> SLKPLTLLMTSSTSFSETINQWADILKTTDMEKFSFDSNPINLLELVKQFNLYVDELAITCEANNVWAKERIDSTPNLFALYDNSGGEAIHGHAFVPYYKESIVLRRLFTVDPNTFNLSRFAAFEGPCQLYCKEHKDSAWVKIQTLLTLGNGIINTLKIIKQAQAFGIDEAVT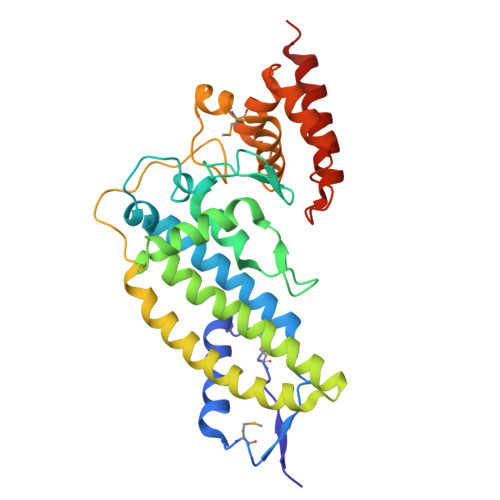ENLKALKEQFIAFQLAEADIKESLKAPSFAEPLPNKESEFFYPIDEKALAKMNGYQLATICLEELNSPKPSPLIERILSNKKFWKRINSAFESGVFKGRTDDPAGKIAKIREWHQLLQISGKKTAG> HMSGPSLQMSLHFSSMDREARVLRYREKKKARK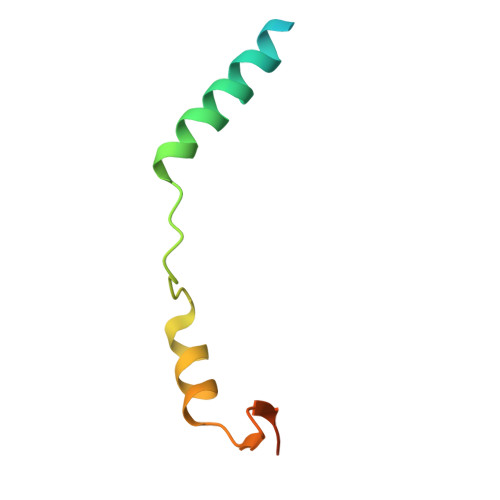FEKTIRYETRKAYAEARPRIKGRFAKRSDVQIEV>EAEAEFGACGAIASTVPNYNNAKLPDPFTFANGTALRTKADWSCRRAEISALIQNYEAGTLPPKPPVVTASFSKSGNTGTLAITAGLSNSQTIKFSPTISYPSGTPPANGWPLIIAYEGGSIPIPAGVATLTYSNSDMAQQNSASSRGQGLFYQLYGSTHSASAMTAWVWGVSRIIDALEMTPTAQINTQRIGVTGCARDGKGALMAGAFEERIALTIPQESGSGGDACWRLSKYEIDNGNQVQDAVEIVGENVWFSTNFNNYVQKLPTVPEDHHLLAAMVAPRAMISFENTDYLWLSPMSSFGCMTAAHTVWQGLGIADSHGFAQVGGHAHCAWPSSLTPQLNAFINRFLLDQSATTNVFTTNNQFGKVQWNAANWITWTTPTLTENLYFQGVDHHHHHH[2x]

A common type of LCC in hardwood is the ester-LCC formed between α-1,2-linked 4-O-methyl-d-glucuronoyl moieties of acetylated glucuronoxylan and γ-alcohols in lignin. It was recently discovered that an insoluble hardwood lignin-preparation (LRP) is amenable to enzymatic hydrolysis by a glucuronoyl esterase (GE, EC 3.1.1.B11) releasing aldouronic acids. WT CuGE has a modular architecture with a N-terminal carbohydrate-binding module 1 (CBM1) domain connected to the catalytic domain by a proline-rich linker region. The overall fold of the catalytic domain of CuGE features a large ten-stranded twisted β-sheet flanked by α-helical elements and a surface-exposed active site. The structure complies with the characteristics of a serine esterase belonging to the α/β-hydrolase superfamily.

To enable structural and functional studies two different variants were constructed, ΔWT, comprises residues 78–458 lacking the carbohydrate-binding domain (CBM1), and ΔS270A an inactive variant of ΔWT where the catalytic serine is replaced with an alanine. For the structural studies, WT and ΔS270A were enzymatically deglycosylated to obtain homogeneous samples, named dWT and dΔS270A, respectively. The structure of the inactive truncated variant, apo-dΔS270A was determined to 1.46 Å resolution. Nevertheless, molecule A and B superimpose well with an RMSD of 0.32 Å for 359 aligned Cα atoms (apo-dΔS270A). In apo-dΔS270A Y366 adopts a unique conformation in molecule B (pH 7.5–8) that seems to be incompatible with substrate binding, but identifies Y366 as a structurally flexible element. The inactive variant ΔS270A is destabilized by ca 3 °C compared to variants with an intact catalytic triad, implying that some stabilizing interactions have been lost, but the overall conclusion is that CuGE is a highly stable enzyme with Ti’s in the range of 72.2–75.8 °C for all variants. The high-resolution structure of the catalytic domain (dΔS270A) obtained from the crystal structure determinations (described in detail later) matched the solution structure.>[2x]SGTEVTTENPSGEELQDP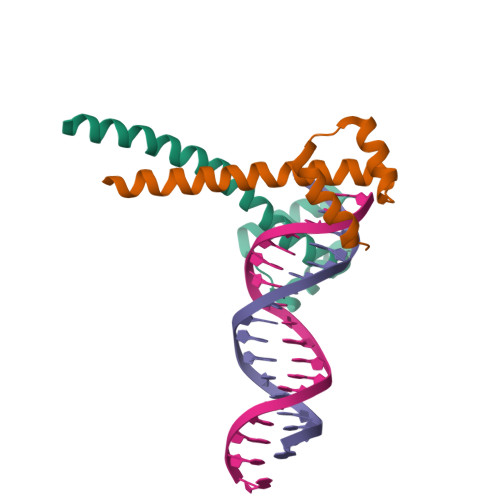SQRPNKKKRYHRHTQRQIQELESFFKECPHPDDKQRKELSRDLNLEPLQVKFWFQNKRTQMKAQSERHENQILKSDNDKLRAENNRYKEALSNA>MEKTTTQELLAQAEKICAQRNVRLTPQRLEVLRLMSLQDGAISAYDLLDLLREAEPQAKPPTVYRALDFLLEQGFVHKVESTNSYVLCHLFDQPTHTSAMFICDRCGAVKEECAEGVEDIMHTLAAKMGFALRHNVIEAHGLCAACVEVEACRHPEQCQHDHSVQVKKKPR[4x]

Microbes use a diverse set of metal-specific sensors known as metalloregulatory proteins to respond to changes in metal concentration in the immediate environment. Zinc uptake regulator (Zur) is a homolog of one of the first metalloregulatory proteins identified, namely the ferric uptake regulator protein (Fur). Each EcZur monomer includes two domains: an N-terminal DNA-binding domain and a C-terminal dimerization domain. The DNA-binding domain (α2–α4) contains a helix-turn-helix (HTH) motif and is connected to the C-terminal domain (α5/β5) using a characteristic winged-helix motif.

The structure of E. coli Zur (EcZur) protein in complex with a 31 bp duplex derived from the znuABC operator (PznuABC) was determined by X-ray crystallography using multiwavelength anomalous dispersion (MAD) data collected at both high energy and the zinc absorption edge and refined to 2.50 Å. Analysis of the complex reveals the HTH motif interacts with the major and minor grooves of the DNA. Figure 1 shows the final model which includes amino acid residues 5–152 of four protein monomer chains (designated chains A, B, C, D), eight zinc ions, and two 31 bp strands of DNA (designated chains Y and Z) in the asymmetric unit. The three dimensional model of the complex shows the central portion of the operator DNA surrounded by four Zur monomers forming a dimer of dimers. The nature of the dimer of dimers ((Zur2)2) structure indicated that there were two possible orientations for the DNA to adopt in the crystal. Using DNA brominated at asymmetric points indicated that the crystal has an equal mixture of both DNA orientations. Given the pseudo-palindromic nature of the DNA sequence none of the protein-DNA contact sites were affected by this lack of directionality; however, several bases represent an average over the two conformations. Anomalous difference data collected at the Zn edge reveal two distinct Zn2+ binding sites in each of the four Zur monomers: the Zn2+ in site A is bound to four sulfur atoms from Cys103, Cys106, Cys143, and Cys146 and the Zn2+ in site B is bound by residues His77, Cys88, His96, and Glu111. Two salt bridges between adjacent dimers were observed, between Asp49 from monomer A to Arg52 of monomer B, and vice versa. Whereas the overall shape of the crystallized DNA is not greatly distorted from ideal B-form behavior (the bend of the znuABC DNA is ∼15°), two of the largest major groove widths occur at bases 15 (18.3 Å) and 16 (16.8 Å), significantly larger than 11.4 Å for B-form DNA. The Zur-DNA complex provides the first structural evidence that the previously identified closed conformations of the Fur proteins correspond to the conformation capable of binding DNA, and further reveals the molecular basis of protein-DNA recognition in the unusually long operator sequence.> MGKKIHARDLREQRKTDRTEKFADQNKKREAERAVPKKDAAVSVKSVSSVSSKKDNVTKSMAKAAGVKSVFAVGNTVYMTSFGRGNDAVLEQKIVDTSHEPLNIDDPAYQLNVVTMNGYSVTGHRGETVSAVTDNPLRRFNGRKKDEPEQSVPTDMLCLKPTLEKKFFGKEFDDNIHIQLIYNILDIEKILAVYSTNAIYALNNMSADENIENSDFFMKRTTDETFDDFEKKKESTNSREKADFDAFEKFIGNYRLAYFADAFYVNKKNPKGKAKNVLREDKELYSVLTLIGKLRHWCVHSEEGRAEFWLYKLDELKDDFKNVLDVVYNRPVEEINNRFIENNKVNIQILGSVYKNTDIAELVRSYYEFLITKKYKNMGFSIKKLRESMLEGKGYADKEYDSVRNKLYQMTDFILYTGYINEDSDRADDLVNTLRSSLKEDDKTTVYCKEADYLWKKYRESIREVADALDGDNIKKLSKSNIEIQEDKLRKCFISYADSVSEFTKLIYLLTRFLSGKEINDLVTTLINKFDNIRSFLEIMDELGLDRTFTAEYSFFEGSTKYLAELVELNSFVKSCSFDINAKRTMYRDALDILGIESDKTEEDIEKMIDNILQIDANGDKKLKKNNGLRNFIASNVIDSNRFKYLVRYGNPKKIRETAKCKPAVRFVLNEIPDAQIERYYEACCPKNTALCSANKRREKLADMIAEIKFENFSDAGNYQKANVTSRTSEAEIKRKNQAIIRLYLTVMYIMLKNLVNVNARYVIAFHCVERDTKLYAESGLEVGNIEKNKTNLTMAVMGVKLENGIIKTEFDKSFAENAANRYLRNARWYKLILDNLKKSERAVVNEFRNTVCHLNAIRNININIKEIKEVENYFALYHYLIQKHLENRFADKKVERDTGDFISKLEEHKTYCKDFVKAYCTPFGYNLVRYKNLTIDGLFDKNYPGKDDSDEQK

CRISPR-Cas13d is increasingly used for RNA knockdowns due to its programmability, but off-target RNA binding and cleavage of near-cognate RNAs hinder its broader adoption. After binding the target RNA, the ribonucleoprotein (RNP) is activated to cleave the target (*in cis*), and other RNAs nonspecifically (*in trans*). Cas13-family enzymes differ in how they recognize the target RNA, but all use two higher eukaryotes and prokaryotes nucleotide-binding (HEPN) domains to cleave the phosphate backbone. Here, we investigated the molecular mechanisms of Cas13d mismatch surveillance and nuclease activation using a combination of cryo-EM structural analysis and quantitative kinetics.

A central hallmark of this structure is a kinked crRNA and a Helical-1 domain that is docked and interacting with the N-terminal domain (NTD). The 5’-end of the crRNA spacer is clamped between the Helical-1 and Helical-2 domains, but the 3’-distal end of the spacer is solvent-exposed and wedged between the Helical-2 and HEPN1 domains. These results are broadly consistent with earlier studies and support a model where the target RNA first hybridizes with the 3’-distal end of the crRNA spacer. In the binary state, the crRNA is bulged towards its 3’-end and makes the distal spacer more exposed to the solvent. Remarkably, the binary, intermediate, and inactive states retained the same overall active site architecture (**[Fig fig4]**).Scribble is a highly conserved regulator of cell polarity, a process that enables the generation of asymmetry at the cellular and tissue level in higher organisms. Scrib belongs to the LAP (leucine-rich repeats and PDZ domain) protein family, and features sixteen LLRs (Leucine-rich repeats), two LAP-specific domains (LAPSDa and LAPSDb) and the four PDZ domains (PDZ1, PDZ2, PDZ3 and PDZ4). The influenza A virus NS1 protein was shown to bind to human Scribble (SCRIB) via its C-terminal PDZ binding motif (PBM). Examination of the SCRIB PDZ:NS1 complexes showed that the NS1 peptides are bound in the canonical ligand-binding groove formed by the β2 strand and helix α2.

We determined crystal structures of SCRIB PDZ1 bound to NS1 ESEV PBM (A281-R219-T220-I221-E222-S223-E224-V225), SCRIB PDZ1 bound to NS1 ESKV PBM (A281-R219-T220-I221-E222-S223-K224-V225) and PDZ3 bound to NS1 ESKV PBM (A281-R219-T220-I221-E222-S223-K224-V225). The NS1 PBM sequence ESKV from the Hubei strain was originally identified via a phylogenetic analysis that identified a mutation in the NS1 protein from the H5N1 virus; the avian virus-type PBM sequence ESEV (which affects virulence) was replaced with ESKV. The SCRIB PDZ1:ESKV complex revealed hydrogen bonds between Ser223ESKV-Ile742SCRIB PDZ1 and Ser223ESKV-His793SCRIB PDZ1. It appears that the conserved His in each domain found on the α2 helix, PDZ1 H793, PDZ3 H1071 and PDZ4 H1170A is an important position even when this was not obvious from the SCRIB PDZ1:ESEV structure, whereas in the SCRIB PDZ1:ESKV and SCRIB PDZ3:ESKV complexes a clear role for this His could be identified. The PDZ1 mutant H793A abolished binding with both the ESEV and ESKV PBM. Our ITC analysis of the ESKV PBM revealed an interaction with SCRIB PDZ2 (KD = 9.5 ± 0.7 µM) as the tightest interactor, followed by SCRIB PDZ3 (KD = 12.1 ± 0.9 µM) and SCRIB PDZ1 (KD = 30.0 ± 0.9 µM) as the weakest interactor. SCRIB PDZ1 displays a higher affinity to β-PIX (3.3 ± 0.3 µM), compared to both NS1 ESEV (21.4 ± 1.7 µM) and ESKV (30.0 ± 0.9 µM) PBMs. SCRIB PDZ1:ESEV and SCRIB PDZ1:ESKV superimposed with SCRIB PDZ1:β-PIX with RMSD values of 0.77 and 0.75 Å, respectively. The −1 position of β-PIX N645 forms a hydrogen bond with S741PDZ1, whereas the NS1 PBM does not interact with SCRIB PDZ1 from the −1 position; instead, the −2 position S223 appears to be the important position, forming a hydrogen bond with I742PDZ1.

> SAPSVKGVSFDQANNLLIEPARIEEEELTLTILRQTGGLGISIAGGKGSTPYKGDDEGIFISRVSEEGPAARAGVRVGDKLLEVNGVALQGAEHHEAVEALRGAGTAVQMRVWRERM;> KMARTIESKV(2S)-2-HYDROXY-3-EPIQUINIC ACID | C7 H12 O7 | 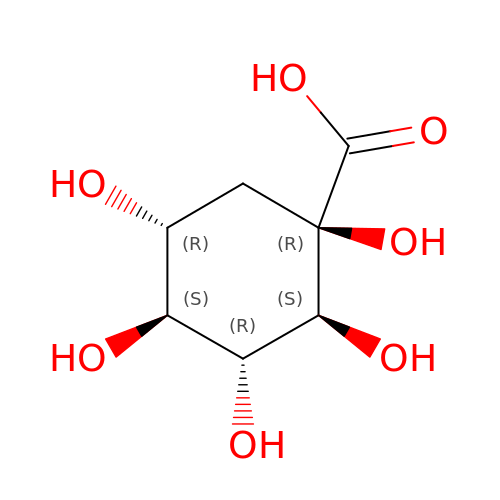OLBQNCISLUABGO-LNHNIDQWSA-N> MSSVDVLLTVGKLDASLALLTTQDHHVIEFPTVLLPENVKAGSIIKMQVSQNLEEEKKQRNHFKSIQAKILEKYGTH;> MNLFWPSETKKQNEIPGGDYTPGNSPSVQKGYQFLNRDIFKSCPRIMERQFGECLHNRTHLIKDLISSGNVGLGPIEIVHMSYLNKHEKEEFGEYFYVTGIEVSGPAMPVEFLEVLKSSKRISKNISNNIILTYCCFNFFSNLDIRIRYDADDTFQTTAIDCNKETTDLTMTEKMWEETFASSVIRAIITNTNPELKPPGLVECPFYVGKDTISSCKKIIELLCRFLPRSLNCGWDSTKSMQATIVNNYLMYSLKSFIAITPSLVDFTIDYLKGLTKKDPIHDIYYKTAMITILDHIETKELDMITILNETLDPLLSLLNDLPPRDADSARLMNCMSDLLNIQTNFLLNRGDYELALGVSNTSTELALDSFESWYNLARCHIKKEEYEKALFAINSMPRLRKNDGHLETMYSRFLTSNYYKKPLNGTREHYDLTAMEFTNLSGTLRNWKEDELKRQIFGRIAMINEKKIGYTKEIWDDIAIKLGPICGPQSVNLINYVSPQEVKNIKNINLIARNTIGKQLGWFSGKIYGLLMEIVNKIGWNGLLNIRTEAFMMETEFYQASNNIIDENGHIPMESRKKRFCEGWLDDLFLDLYQDLKLSKISLSNKDEKHSGLEWELLGLIMLRTWHWEDAVACLRTSIVARFDPVSCQQLLKIYLQPPKNIQEVTLLDTDTIISLLIKKISYDCRYYNYCQIFNLQLLEKLCNELGTHILRNKILLQPSIGDEIMVMIDAMLAWIADLDHTVQPGTENLYFQGHHHHHH;> DDYYLNLNQDEESLLRSRC

One of the many transmembrane proteins that follow this route of transport in yeast is the chitin synthase enzyme Chs3. The transport of Chs3 to the cell surface requires the exomer complex, which acts as a cargo adaptor for Chs3 and other cargos. Exomer consists of the core protein Chs5, and four paralagous adaptor proteins called Chs5-Arf1-binding Proteins (ChAPs): Chs6, Bud7, Bch1, and Bch2. We also present a crystal structure of a portion of the Chs3 N-terminus bound to the exomer complex.

After screening many crystals, several were found that contained the peptide matching residues 10–27. This peptide formed an alpha-helical structure, and bound to a region on the surface of Chs6 roughly opposite where Chs5 binds. The Chs3 peptide makes direct contact with several residues on the surface of Chs6. Chs3 residue D19 appears to participate in a hydrogen bonding network with Chs6 residues D731 and R713. Chs3 residue E20 appears to hydrogen bond with the main chain carbonyl oxygen of Chs6 residue G31. Both of these Chs3 residues, D19 and E20, are part of the conserved DEESLL sequence that was previously found to be important for interaction with AP-1 and that we found to be important for endocytosis of Chs3. Interestingly, the conformation of this motif when bound to Chs6 is alpha-helical, in contrast to the conformation (D/E)XXXLL motifs adopt when bound to AP-1 and AP-2. In those interactions, the (D/E)XXXLL motif is in an extended conformation. Nevertheless, the structure reveals how this clathrin adaptor motif can be bound by exomer, perhaps providing a basis for competition between adaptors at the TGN.> SSQIRQNYS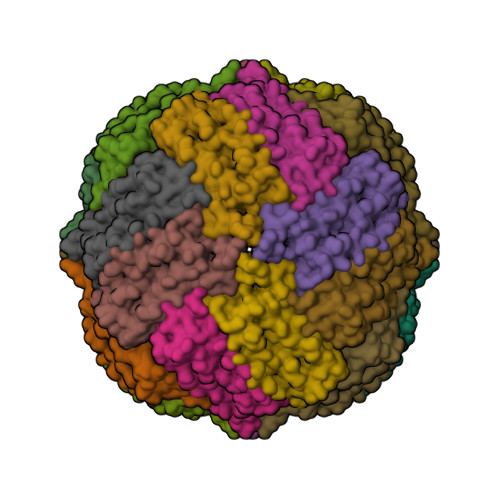TEVEAAVNRLVNLYLRASYTYLSLGFYFDRDDVALEGVCHFFRELAEEKREGAERLLKMQNQRGGRALFQDLQKPSQDEWGTTLDAMKAAIVLEKSLNQALLDLHALGSAQADPHLADFLESHFLDEEVKLIKKMGDHLTNIQRLVGSQAGLGEYLFERLTLKHD>[2x]MMKPEDVIKEQCARAKVVAELWHGFTGGAPKAALENLVVEFNKAQQGRCVRPVPQGGYRDLSTKIKAAFAAGKVPTMAQAAENNIALYLEAKALLPIESLGVKLQGVNLTFLNAVRFGGVVYGVPFNKSIQVLYYNKDLLKKHGVPVPATLEEFVAAAKKLSRAEGGPVYWFQPDA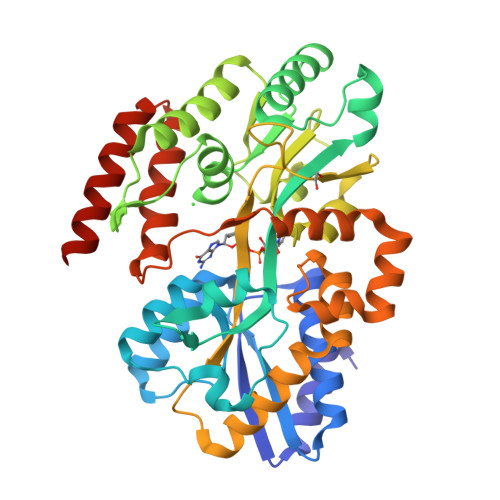STFAYFFFNLGGSYLKDGKLVLNSKEAVEALTLLQNGVKEGWAKPITSGYINQNLGSGPYAFSVDTSAGYTYYLRAAKFDLGVATLPGRTKGQPGYGLVQGTNLVVFRQASKEEQAVAKDFLEFVLSPRAQAVFATATGYVPVTEGALKDPVYQAYAAENPDYATIVRQSRYAKFEPALAEWEQIRFDILGQAIKEAILNKADPKAALDRAQKLAEDLLSSRTRHHHHHH>MSGKEEIKEAIKKAVVRARVTGDPKYLEEAKALLEKLKELDEEDKDVEKFEKAIKQVEAELTLKEAKEVVKRLFEEGRPEDAAREAFEYLQKLLDIGSPEAVKELLQ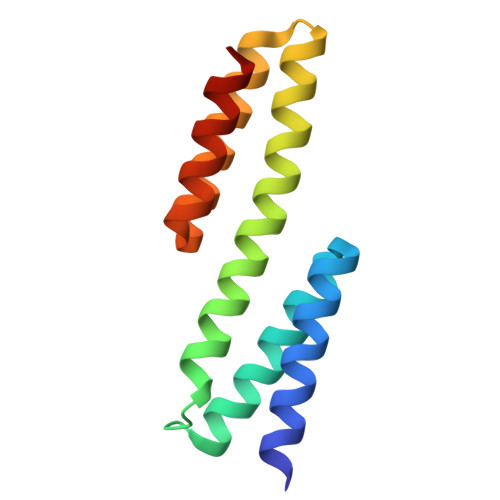FLRELLGSG[2x]Central to ERQC is the ER-resident 170-kDa enzyme UDP-glucose:glycoprotein glucosyltransferase (UGGT). The enzyme selectively reglucosylates a misfolded glycoprotein on one of its N-glycans and promotes its association with the ER lectins calnexin and calreticulin, thus mediating its ER retention. The full-length Chaetomium thermophilum UGGT (CtUGGT) crystal structures revealed four DsbA-like domains (TRXL1–4) arranged in a long arc, terminating in two β sandwiches (βS1 and βS2) tightly clasping the glucosyltransferase family 24 (GT24) domain (Roversi et al., 2017). Overall, UGGT's motions can be described in simple terms as two rigid groups of domains moving with respect to one another.

To assay the contributions of individual UGGT TRXL domains to UGGT reglucosylating activity, we cloned three mutants of CtUGGT, each lacking one of the TRXL1-3 domains: CtUGGT-ΔTRXL1, lacking residues 42–224; CtUGGT-ΔTRXL2, lacking residues 417–650; and CtUGGT-ΔTRXL3, lacking residues 666–870. CtUGGT-ΔTRXL2 and CtUGGT-ΔTRXL3 expressed and were purified. CtUGGT-ΔTRXL2 also yielded crystals, enabling crystal structure determination by X-ray diffraction to 5.7-Å resolution. CtUGGT-ΔTRXL2 and CtUGGT-ΔTRXL3 reglucosylation activity assays against urea-misfolded bovine thyroglobulin detect impaired reglucosylation activity upon deletion of TRXL3 and complete loss of activity upon deletion of TRXL2. In contrast, CtUGGT-ΔTRXL2 is completely inactive against urea-misfolded bovine thyroglobulin. The total loss of activity of the CtUGGT-ΔTRXL2 construct in the reglucosylation of urea-misfolded bovine thyroglobulin also points to a critical role for the TRXL2 domain. The CtUGGT crystal and cryo-EM structures (Roversi et al., 2017), and our MD simulations, all highlight the TRXL2 domain as the most mobile in the molecule, supporting this hypothesis. In the light of these data, it is possible that TRXL2 motions adjust the size or vary the surface area of UGGT's central saddle, making the bending motion a crucial one for activity against this substrate. Our observation that the face of the TRXL2 domain overlooking the central saddle bears distinct patches of hydrophobic residues conserved across UGGT1 sequences (Roversi et al., 2017) supports a model of hydrophobic-mediated misfold recognition. Our data support a “one-size-fits-all adjustable spanner” UGGT substrate recognition model, with an essential role for the UGGT TRXL2 domain.

>[4x]ETGQVAASPSINVALKAAFPSPPYLVELLETAASDNTTIYYSLLDRIAKGHFAEATTDKALYEKFLEVLRDDGHMDPEALSAFKLALSLRTATPRVEAHYQYYTATVEPSLSGTQEGCDQWFLIDGEQYCSPTLDTSHGKVKGEDQLRTLPFDRKFGVGSRDVILYADITSKSFAPFHEVAMDLAKKGKASYRVRYRRSPSHSRESLSVNGYGVELVLKRTDYIVIDDRDTGAAAKPAEENDQKPLVGHETVLDDGEEIADIKPLEKSELAALGMKAASFVMQSEKPFEALLKLTQDFPKYSNSLGSQNVSAEFEAEHRGNREVFLPEGSNVLWLNGLHLIDRQIQPFGLVDLLTRERKLIKSVLDLGLTGQQAVDLLGHAEVAHAKSGDDEPRRFALSRRNTLIFPEDKNELTVLNVNKIYIENHDLMSKVPVIEASKESTRDDWAALTVVADLDDIEGQELVYYALRFRKSNDGVRLDIVHNPKDTSRSPSVLAQRLKSREDKLLDFTRFLDLETALETGEFEPDVAYDASLANFLASSNMKAGDNFVILNGRVLGPITSADDFKKEDFEVFLQAERRTRILPVYKALEDLGLDDKVSGPLSAAKLTSVTALSTISDLPQGIFDNAPTVRTTLFKQWNSTYTSFEVGDASTATIFFVAVINPASEIGQRWVAVLKVLSELEGVHLRVFLNPTVMIEELPVKRFYRYVLSSSPSFDESGKVKALSARFTGVPRETLLVVGMDVPPAWLVTSKVAVDDLDNLRIKDIKAKRGTEHVEAIYELEHILIEGHSREIPGAHAPRGVQLVLETENNPHFADTIIMANLGYFQFKANPGVYNIRLKEGRSSEIFTLESVGAKGWGPIPGDDNTEVVLMDFQGTTLYPRLRRKPGMEEEDVLEPSTKSGEESGSGARNLVSRGIKFAEGLLGRGNKAAEATKSVSKTEHAEINIFSVASGHLYERMLNIMMASVMHHTNHTVKFWFIEQFLSPSFKDFIPHMAAEYGFKYEMVTYKWPHWLRQQKEKQREIWGYKILFLDVLFPLSLDKVIFVDADQIVRTDMYDLVEHPLDGAPYGFAPMCDSRVEMEGYRFWKTGYWANYLKGKPYHISALYVVDLQRFRELAAGDRLRQQYHALSADPNSLANLDQDLPNHMQFTIPIATLPQEWLWCETWCSDETLKDARTIDLCNNPMTKEPKLDRARRQVPEWTKYDEEIAELARRVREEKPKKKEEEKVQKNPKSRRLDGDEEEVKTVREGTKHHHHHH>[2x]MRVPEKYSTLPAEDRSVHIVNICAIEDLGYLPSEGTLLNSLSVDPDAECKYGLYFRDGKRKVDYILVYHHKRASGSRTLARRGLQNDMVLGTRSVRQDQPLPGKGSPVDAGSPEVPMDYHEDDKRFRREEYEGNLLEAGLELENDEDTKIHGVGFVKIHAPWHVLCREAEFLKLKMPTKKVYHISETRGLLKTINSVLQKITDPIQPKVAEHRPQTTKRLSYPFSREKQHLFDLTDRDSFFDSKTRSTIVYEILKRTTCTKAKYSMGITSLLANGVYSAAYPLHDGDYEGDNVEFNDRKLLYEEWASYGVFYKYQPIDLVRKYFGEKVGLYFAWLGAYTQMLIPASIVGVIVFLYGCATVDENIPSMEMCDQRYNITMCPLCDKTCSYWKMSSACATARASHLFDNPATVFFSVFMALWAATFMEHWKRKQMRLNYRWDLTGFEEEEEAVKDHPRAEYEARVLEKSLRKESRNKETDKVKLTWRDRFPAYFTNLVSIIFMIAVTFAIVLGVIIYRISTAAALAMNSSPSVRSNIRVTVTATAVIINLVVIALLDEVYGCIARWLTKIEVPKTEKSFEERLTFKAFLLKFVNSYTPIFYVAFFKGRFVGRPGDYVYIFRSFRMEECAPGGCLMELCIQLSIIMLGKQLIQNNLFEIGIPKMKKFIRYLKLRRQSPSDREEYVKRKQRYEVDFNLEPFAGLTPEYMEMIIQFGFVTLFVASFPLAPLFALLNNIIEIRLDAKKFVTELRRPVAIRAKDIGIWYNILRGVGKLAVIINAFVISFTSDFIPRLVYLYMYSQNGTMHGFVNHTLSSFNVSDFQNGTAPNDPLDLGYEVQICRYKDYREPPWSEHKYDISKDFWAVLAARLAFVIVFQNLVMFMSDFVDWVIPDIPKDISQQIHKEKVLMVELFMREEQGKQQLLDTWMEKEKPRDVPCNNHSPTTHPEAGDGSPVPSYEYHGDAL

Calcium-activated chloride channels (CACC) facilitate transmembrane anion conduction in response to the increase of the intracellular Ca2+ concentration. The most prominent CACC is formed by TMEM16A, which is expressed in different tissues of the human body. Structures of both functional branches have revealed the general architecture of the family. These proteins form homodimers with subunits containing ten membrane-spanning segments. Our study reveals the location of a hydrophobic gate at the intracellular entry to the neck that controls ion conduction in TMEM16A thereby contributing to the tight regulation of its open probability.

To characterize the structural relationship between residues constituting the gate and address how their mutation to alanine stabilizes the open state, we studied WT and the mutant I551A by cryo-EM. We next investigated the structure of the constitutively active mutant I551A in the presence of Ca2+. Although at a lower resolution of 4.1 Å, the general correspondence of the mutant structure to WT emphasizes their equivalent properties in the Ca2+-bound state. Whereas the mutant resembles WT in the Ca2+-bound state, the Ca2+-free structure of I551A exhibits pronounced differences compared to the corresponding structure of WT. Sidechain truncation of any of the three residues by mutation to alanine causes a strong increase in the potency of Ca2+ and results in pronounced basal activity.>GPNCAPGQKVKLFRASEPILSVLMWGVNHTINELSNVPVPVMLMPDDFKAYSKIKVDNHLFNKENLPSRFKFKEYCPMVFRNLRERFGIDDQDYQNSVTRSAPINSDSQGRCGTRFLTTYDRRFVIKTVSSEDVAEMHNILKKYHQFIVECHGNTLLPQFLGMYRLTVDGVETYMVVTRAVFSHRLTVHRKYDLKGSTVAREASDKEKAKDLPTFKDNDFLNEGQKLHVGEESKKNFLEKLKRDVEFLAQLKIMDYSLLVGIHDVDRAEQEEMEVEERAEDEECENDGVGGNLLCSYGTPPDSPGNLLSFPRFFGPGEFDPSVDVYAMKSHESSPKKEVYFMAIIDILTPYDTKKKAAHAAKTVKHGAGAEISTVNPEQ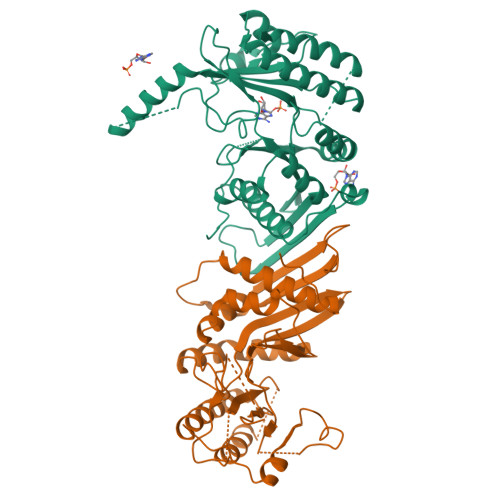YSKRFNEFMSNILT[2x]>MAKPANKLVIVTEKILLKKIAKIIDESGAKGYTVMNTGGKGSRNVRSSGQPNTSDIEANIKFEILTETREMAEEIADRVAVKYFNDYAGIIYICSAEVLYGHTFAGPEGASAWSHPQFE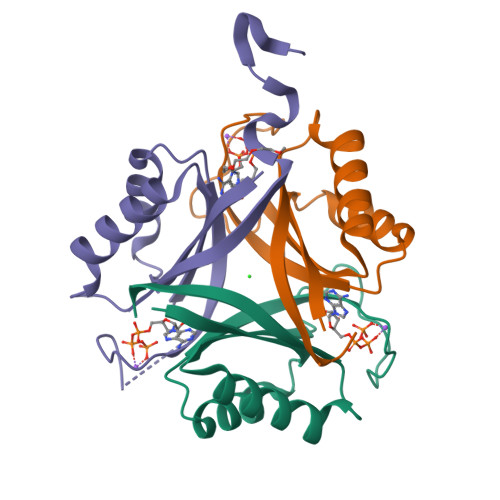K[3x]cGAS has emerged to be an essential protein for the innate immune response to cytosolic DNA given its activation of Sting by the production of cGAMP. The generation of cGAMP by cGAS requires that the enzyme bind to dsDNA and use its two substrates, ATP and GTP, to generate the cyclic dinucleotide. Our previous structural studies have shown that upon dsDNA binding, cGAS is activated through conformational transitions resulting in the formation of a catalytically competent and accessible nucleotide-binding pocket for generation of cGAMP14. Here, we report the discovery and characterization of a class of compounds that binds to the catalytic pocket of cGAS and inhibits its dsDNA-stimulated activity.

We were able to solve the crystal structure of RU166365 (hereafter as RU.365) in complex with cGAS and dsDNA, allowing us to better examine the structural basis for the affinity of this inhibitor. RU.365 occupies only one side of the cGAS pocket, as does cGAMP in our previously reported structure, leaving the remainder of the pocket filled with solvent. The benzimidazole ring and a part of the pyrazole ring of bound RU.365 partially stack between the guanidinium group of Arg364 and Tyr421, which represent the key intermolecular contacts between RU.365 and cGAS. The angle between the pyrazole ring and phthalide ring of bound RU.365 is approximately 120°, which is mainly caused by the interaction between Cys419 and the hinge region of these two rings. The remaining parts of the phthalide ring face the solvent and form no interactions with cGAS. The benzimidazole-pyrazole and phthalide moieties of RU.365 overlap with the adenine ring of ATP and the α/β-phosphates of GTP, respectively. The entire RU.365 molecule overlaps well with the AMP moiety of cGAMP, with the benzimidazole ring of RU.365 inserting deeper into the pocket than the adenine ring of cGAMP. There was not a large difference between the affinity of RU.365 with and without dsDNA, both being between 64.1 nM and 98.5 nM, respectively. We found that the affinity of RU.365 decreased in presence of GTP or ATP (64 nM in absence of GTP vs. 298.2 nM, in the presence of GTP, 104 nM Kd in the presence of ATP). Taken together, RU-365 appears to impede the binding of both GTP and ATP to the enzyme active site.

> KLKKVLDKLRLKRKDISEAAETVNKVVERLLRRMQKRESEFKGVEQLNTGSYYEHVKISAPNEFDVMFKLEVPRIELQEYYETGAFYLVKFKRIPRGNPLSHFLEGEVLSATKMLSKFRKIIKEEVKEIKDIDVSVEKEKPGSPAVTLLIRNPEEISVDIILALESKGSWPISTKEGLPIQGWLGTKVRTNLRREPFYLVPKNAKDGNSFQGETWRLSFSHTEKYILNNHGIEKTCCESSGAKCCRKECLKLMKYLLEQLKKEFQELDAFCSYHVKTAIFHMWTQDPQDSQWDPRNLSSCFDKLLAFFLECLRTEKLDHYFIPKFNLFSQELIDRKSKEFLSKKIEYERNNGFPIFD> MFLIHFVHYKTILQKYTFKFKHIFLSIDKYNSLFFNISGILIWLNIIHINIILIKYSFFILINNFEYLIILIST;> MFRLTAASQKNLNSWYTKGTMRGGVPRIYYAWMRPGSFTRRRFEKMRNPFVDLETGTSLYFRDTRDSAEAIAHAADSKGIKGMDNAIDLYNEYRIVPDLYPEGFQWKHKLNTEYNQWRSNTWLTPDLIPKEHRGRFLCNFQLNIVAYDMRVVKFSPKDHRQWIYCVLYVGSGKGIAGWGRAVAPSTQEAKKEAIREAFSNIIAVDLEQEGPMYPVRVNADGVRVLLYPARRIVANFRVADILCAFGFQHAGCRINLKATNNPKSPTHTVEGVFEAVKALRSVSEIAASRGKVPHSLIYNIYPYLEEIRRRKGMMAMHPPGKDGLLMPDRVVDNRLPDHLKRGYYDDVYWKDFFAGSDEHLNEPRMGLRGDEMRRRLEEAQTSPAPTTAKDTRRRTLEDVLKRLGKTTRDLGSIPIVNPRVDVGLPTHIKRNYQLH;> MVFYSFVLVMKPRQRRFTSQALREIGVAVYSNGGLIRSITNEGIMRPYSRFRDADNTPLTYARYIILQLDMGEEEMGKVDKIIREHQDVLMALKLNNLERPVGIRSGNKELQAAYFPLDTFTRLEEEINWSPQTSADIYTQLEMNWKEFSRTRWSSFLRN;> MLRQSLLSLAKVYGAVPPLGAAQGHRLLHGKREREGSLFAVANDVKRDERLLRQQLNALLEEERMPMQARLQRNEAVSSHEAVPQTPLVDLPGVERRRDLPADPITRLFFQHKGDHALYYGTYDKPSVQDDDRVQIEKRVPRRREENLYTPIYDFCHRIREATEQRKRFVVVPSTIETRGCARVMHDHGLVAGFRDFHNDRAFAVELKYFQGDSTINVIEPCSYDGRTEFEWSPKMMRRLLNTHGIHNRLVVYICRTADNRIIDHIHAVKENIGGRGLMMVH;> MQKLLSPRTARHARLFRLAGKLADSGSPGVPKSDGERLVWVNSHVRRDKDISLSQEEERIRELMMPLEVGENSFAANGQATHGNLFYFREYPMYPGEYVPAEHNTLSSLRDELRLDLTAQSLKEAWMRVSGGVYFQSVDEYYASVDGLDAEQIGEVLAALFPELNCYEAQALVQRTLECISRPVSAASRQLSRTITAEAVGLDNAPGHYTNFLEWMGRLTETRAFKTEHALFEFSRRKFNRDDVRVMFENYRLMSKATLLADSADSYSHFYTVLKDFARKVAGEDSRHQIGVRIDEAEVDPETGIAVGRGCADGEKYHFTALLRENRDHNGIITVMGKPLSLVLDNKAWLMEMVLMPFDEANLDYRDFDAHIVSEGHAMPSIANEIAAFALRMAVANALVKLIPLTRIPLKKSGLLSVDRRRERGQFPGYLDGKKVKRRFAKR;> MVRRSHVVAYYWSRYRMPTQMPKFDGPAPVAAPQSMNSTKTNEFIDPIDDKFPMSIRGPLVRPDVPEDQYVDSWYICTSMTHHMGDYRPWSASAPPNAFRFRPFNEFDAKGREYVQYMREFARFDPRKSRGNGQKGFPFRDAYLTKMNEANQKTPPPTLETIMDRAVREHHQHARILSPLEVQRDVGRLEPIPSYAGKINADRSVFPFQWKTEDWYEYEVAKVRNRRFVFENTEEDGIRGSEVTYKIVLEGFWDHHVMKLAEDVCMFLKDVGRQIVEEKLVAVRRLLQGGAVDPELLAAFNCARAGPFGGLDEYDKEEVANFLRSDLRRLEEQCLSVINRCNVPVPGATNIYDPHTSWPHVEKLEPWVRMAEFWTSSSDTSFTELEMSTAHYEFRKFFRVIICKLPFQSTEFEKRMYDIRHWLHRQTSCEFHTIYRRNVIHDSAVFPTEHDPATPTTHEHHRMFSFALDWQSAPVNRLSTDTVHEGESWDAVAQRLGCSVGELKDANAERETIEAGVVINVPVTATRRLTSFGATPLVLPLKTTSAKDGERIRTWEEAAAILDCTVEELQQCNGHAALTYQKKESEAGEFDSSVTELVAPLSCWTSTSESEFSPVERVHANDTLVAIARRLQCSEEALRAVNDGITDVSGLDFVRVPPEARRPRRLVEPQLRPQAATDALLARTIAEEETFKLKSIPHLPQNAERFPHEYHTPTSRFPPTPSETPATQDWMAYTAKYLDKQFTISAEPAPVYNVNKLWPMQQIPGKVDQTPFEEDQTWLLHSIPVQQLEMHHHEKDLQDLPFINHEQFPRSLEWNAP;> MMRKSVTFLRRGKPRPRAGMFPDKYRRVPMLLKPQQGGQQYFNHFLIRSTNDRLTQQDVDNASGQAHSFISPQLPQMDWRNMSARSSEESIREEMRQLAENDVMQHQRVFNERMWYEKEEEHRMKARSCPEETSEHAXSNDGAVPPPRVLGGDYFKTRFGYSLVKNSEMTQGPVDYSQLDMWGEMPRYTSDMVFLYLVSRRRNTYAVAYTYEGKRILNTYTAGNRGLKGGDRGFRSEGSTDNGHQVTSMYLNDLLPKLREMRASEGRPMGRGEKVELVVRVMGFYNGRQGAVRAVQDRANEFHVRYFEDITPFPLNGPKMPRGVFK;> LFFLRMWFLYGCCLRFVLFVLCYYMSPRLPSSGNRRVLYAVFYLYNFVWMLRCFFCCFIGLVMSLFIIEGGGFVDLPGVKYYTRIVS;> MFCFSRGLWMRHIGQDVPKRHTHFVLESRLMYEKSFRDCWLHSVCRAISQLDEPLSKTVVGTHQKMLQRKVTCFQYNQYGLFKTPYYRLANVDRYHAVQGVAGTREWVPYVNVSYWTMNKMVRGGNLLVHRVHYTGWGTDSHLKKGGWEHRWNKVLQRNVLQYSRI;> MFVRSFCFLRKYGSKSKTPDLKTSFTKTTNFRKAEKISITTTDGEIVKGRGKIRRRTHSALKEAIGAMEHPAIWLWYPWRMNPEPPTPHMPQRRALKNVHGAVFNDLTPVQKKRQEQMLYGVNIPETRQMKFEEQHPLLAGALRKLEGQPKGFPFWYRKYPTRRHAYEYRFSIPVEMLDGYNDDVKKALSKGMMSIQEKQFAQEAMYMERYAEHDFDTTSPAVLAVKRALKCRVLRNHLLTNPHNNIIKTVLANTERKLNHALRRLRKVDFKKYWEIIRDHDVQDILQPPNLVTYRQGSYWKYDWNAGLAISTNLADVMDPRGLNGCVETGRSRSEVARDLGLSYTRPLHENEKKQLSHQAVYYERLAKFKMEQPEAARAMERERFVRKFSGMFVKMDIRSGAPDFPSTYRRLLGTKVVRWASKRHGPN;> MQVTETVLARAVIKRRSPQLWGAPGAPIIRMRGHHVVWKFQSYDLVVEHTHKRRNSDIRLLHYLGKHCPHPQKSLWSPDTPVAQDRHLFMLTTVDIDAFKYWFGVKRCRLSMKPWALLAKAGLLPPSLTQNSKIMPKPLFDKESLMRYYLANRKDEDVMAREKYLNYENSMVKTEEERAAERPVAPYL;> MLRRSLLAFPWWNFQTEHRQRCVLMYGGARTKNTHNANHRVFIKKYKRNAFPNRTRHHWAVSMTGVLSQRPRRMPWPYDLTSLIFNQPRQGSDKIGYVVGTSMLKTAVVATNHMVYYPKFNQRVSRTKRFFAHDEDLACVEGDLVHIKQCRKISKYKHYYVFSILEPNVEGRERLKLGLKAVPPPLFGYPVSRRIVKLNLTSTEGTQEKLAAAIQEHVQDAYRFSGPTPDQPRNRLADPVTFEDANNMIAPNAPAAAALDASDSPPLLDRGEYTEVEQDTRNKKGDDYWMNLQPKEKYDFKSFKKSP;> MNRTGGSIYAHALSQFAVCRQPWNEYIGLLTKQDSTPYHTEPQEKPAYRGRKQGREGWLFGQQVQLHYHRFPDEQLITNLSRWRTGETVGDIAMQQFRNAQPFDIEDKDPQGVQRPSPEVYMKLNYKNPATISRFLTRTGHMYPADILPLNPEAVVKLRVAKAQAIRIGLYPRFGNPFWFRSQKFRPKAYQENYDPTTYSTKRTVEHFAYNWVQTDRIRRYFRELEAVHTSGSASARGSGGGTTAEHKQQDQFYSPENQPISLHRNNISYMEDVGRSVKNPTVPGLMSTKGMKKKFHNLYSSTSTKRMGFSNPTLGIKKV;> MAFRNTFTTPGKFSTVSKNIVLLLIWRVKVFLRAEGFAHSLVMLPVSLYSKILLCDVKKKIVYFHCCTRKKSMLRRCPCVWPDGPTKSSVSIGTAFTLQKRFLKIAKSAFGFYLARRGQRKYPFLRRPHIKNTHSMNPSAPYFWSFMTAKSQMAFLPEENYITGDWTGKFFVSKRQVYTLQHATSGAKVRVKSFPSIFEFNSPSRWNIGKEMNTLTKPRMDLIDEQMLTKKQRLDYVRAGLLPK;> MLHTTRLWLGGYMMYHRKAMGTMKYSKWKGAHGGISHFYGRTPMVEEVRPNEPITLVDRRIMHYVHHSRLRHFQLFRSYQEKSNSTECKLREGEMLRRRWHRRLQKSFIAFMQFKTMKVLEDQARLVNTYGQAAVNAALGDPWNATDNVARERKSAAVRRQVRALPMVNVVPKHVATMKQIHNDRFNYRWRVN;> MLRRAYIQRRYPFNKRGPREHKSWKHHVLTEPPKPLQWRDPKVWTRDLSVMKSFDAPQWDLWQSRPRSEDMDEALQPFMDMPKSLKDRRYDIPWWANPFGAWYLQNILSLELLKLKSKTNAEKIATYRSYMRSLASGKDNTMSDDDVIRNIIKERWKTLEFGDRNAGYPCTFGDYIQFLNEWFKSLDEEGMQRLREHFDRRIRPLLAVMSPVDILWLEALTQNSPHNKEQLQRKIAFQTSLGTPEFFDMSKRLRYEINEDYKVRDELGPELFALWSKAPERWPPERLSKMYGLDFTLVRKILVWHHFKACYDACVEPDWSLPKRLFALEWIRDVRARKHGLFYGKMRFAEQKITFYSDRFLFRDLVNRREASYANVWEMDDPYRFLQTEQDYEDYWGDNYDVYRRMFPEMIGRTGEPVQQYGQMPIWAGPHRQHANKSEHNWMFAEIGVNVGHEALKKLELDPTNEKRRRFVIRQPDGTLRSAKMSEMRAWYWKEEWADFRFWAPQMEWGIENTPSQEQYQEHVPDTTDADFRKQRRIQSRPVKWFYESHYTRTGSFAGFQPLRFMQRRTEREVRWPDVINAAVQIQKRKPAAYIFKAIPEL;> MRQCVVRRYKMPKNMGVAPRFDTWNEKYEPWEHMKRMGRLVGTGFYIPPEWYNHFRMFPPINHNFQQEKTLNPHNASEPTQDDTSTLSPERVALRDELARKSRLVASEGMRYYNIFWVRKPLDTMEKEYYELKRRGVDHGEAIRKVLQGFYSGLAVKKRVAAIQAEEAKLTGRFITMREATVVLGVLAKLHKEQLTPHQVSLLAKEQGETTQSGAKLTAIVSRTQPHVNKEASSPATSEAVGSSTEESLSADALASMLSEDGEQSAVGTRYQVEVKETANDSVRQLREKAEDQTGFPDWYTGESPTYSGTSXCSRDGFALMKANK;> MMRSSSFCRRQIRPYYNLPSKSEHGRKMTGFLTPYRHWMWKQNELWRNVHEAQFEHLRRVYKRQWLESFRVNADEYIYKYNITKAAQLAQWECEMKEQEKKRIEARQMMDGRQALKKKHLDLLREFHERQFFFWYERASERLQNMNLINYVPHAQLREHIDKELDKYVAGKNEPYPLNFVGQMPFLEDGDGNIVEVPESLLSNHMAEHPDSTAKPHEPHTSSSISEAAAFEERMLRAMVSAKEEDLKEWLGDDSRALSETIDDISREEEEREADIRVARSMEETDAEREVSRRAYIERXKTGSRSIFRPPTVSEGAGGTPSAPAGDANTPMRRRKKGKLDRVHALQAHQDELLAKLSSQGLKEXVDASSVPERGKIVQSRGRIRDKAVIPTHEVLMQKPELAAGSTPGARIQTKDMVDKMYHRGKYKKSGSGDKSDGEDL;> MRSKTLKKSLAAMYMRPPVTCYTDACEAPVAMWDGAIPLKETRKLKNGVPVRTVSRTYSHPPQLTPTQLSFNDINSMYCVGNDELIQFFPEGLGGRVFQTMPPGHPRGFLYRKETHLLNLFVDKVQHWHTKRSVLSSLTNGRTGFIVDGPTGCGKSALMCQVVHFARSRNIVTLYVPDAKVWTHGEWCWPSTILPGFFDAPDAARSFLKYFAVANRATLTSWKLRCTPKDLPTEQGERQPQNLYELCEWGHRAVAPASIDRQSVCVKFLMDELSEEKKLPVVIVVDGWNLFSHETHFRYPHPDFLRGLASFNESSTDIDLYPQELPRIPASRLSFVRGLNKMILSGDDPNKFFITCTTRDFKPFDGISGFPNVETDRFANSLDEYAPYDPEKDSHFHPIQIGNFDEYEYRSFLRFLINSGELAGLGWGPLWHASSDFERKLYKIGFLSGRNPQGVVDHYHQELVWRYDYQRTRQKQYLLKRRMEGMSRGASSGAVGVR;> MVLRRWFPLLGVHRVGYTHPSTLPVPCAQRWDLRLARARIFQEYIEEKAPGAWQLEDERSMSPEFKTFTGYPMRDMRPGYGQNLPDYIMKKRLPNNTHYELFARRDIPNEDNAMYGKYLYDMTVHGTSLPSTYRMHKDINKAQRNDRKLSGNRFKVLCSSGAKNPPSGWEPIPDATEEEED;> MLRCARVALRADPLNGGSSMTLGSKGSKLSPEPHRRRMPWTAAKEYVPGVVLNARDKMVLDGVQLLDIESIDRASQLDPLEVLRAVVATREYNISTGKNIFQLASQATYNGRGQRFYRKEWQEGTYDKYVTLSAIDFDRDGNKGTAYGYITFHGETTTRPVQVDFADVPGWYMDFVEERAVPFTGIVPPPPSIGTDVPVDPHSYRLKAYPYYDAPNPPEFVERLLKDRGVLPDTPTETADVDKDPTTSDGSVHYDGK;> MRRWHRSLNPALFGERGSGHYFSTTRARLQLQAQDRIICGTHGAGIVAHQTAVNSSDNPMLSSVTTAAPAADLSRTKPHEGTGTSERDPYIRTLHNQRSAAPESSVSQSHTVNAPTVDECEMLAERWGTMNYWHNDTFPRLVVFLKKLLVPDVSPLSPTAESLLSMFEKVVIPKLTSDEEDRRKLVSLWSETTLQAEAAVTKFLFQRGSFESMLHRIITDALEKMSTLALGGQEGNLALEALKRQTLFKRNDYIQKRLIDVVSNSAYLGYGDSVWQVFFAAVEANEENLLSDRATTDAIRAAWEGVMREDVVRLPDVTGVVALYLTLVCIRESGRLVPEELKELSSGLEDGVRPGVRKLQQYPLIFLHPTVKRRFVVKAVAEILHNSSSNAFSNMLRENGLHDTAREVALCEAMNRNKELAEGDVGDAVGRFVSKGEVKTLLSSLVSGTDAVVRDAVAGIFGIGTTITIDWDAVMQNVDWSNNWQRLATALLSNSAVLSAIVKLVKNAIGAKGMSKHLFTDEYADQLQLILDAREERAASRKQRIENIAQELSSFERVDLSCDLLRKLGVDMTELDTAAAATRNMNVVQRPCIEDGLLSLVLEAVTKRHPNWVKAGVIQTTLKDPFDALRWMMHIFIRLSYVPHAGAATIARLSRRRIGPIGLEPHQFNVPAELGFVEQYDNLQYKRYDWQGWYQRMLDVHNRNVSLRCRICDLQRLDGNGVQFVDMQTERRLRILAQHRVGMGVLKLDADKYEDQADNVTFGTTKLSELLADARKAQLGEEYWPSVELKVRKPSGQSKAHYSLIDNERIEKRSGELYEKYRDAKKRSLFVTPMETWLEVKGMQVRKSVDNADEDGYTLDALQDMMDGDDGDKV;> MKSSDIFFAYRLTPVVFKSRQHDSGVNQYGLKPTNAYDYINPTNLINFGRGTTFDNLGVRRAGRGEIDSSPSHSGSPVFTQAKLIGLSGEEQLTMCQSETMALRLCMAKAGKETCERESRALDSCLGRVGHLRRAMSEACWEFNDWFIQNVSDNHTKPFQHRPHDWRHFYAQEKLVRERQQNGHAYGRRPKQFSFGARYVKTDGYGKRPRLPYNK;> MRAGCVACSRIPKLGIAALGSTTTSMQATCQETQELRCATTQMAPAVIFPLPPPLRGSYIDRKPTAASFNEHHATASFRHHMIASADVSHRPRHFYFASGTRNDTGTRSVKEGERKQLKQQTNVEVDSVAYGDQLDELSARWAAKFYGQVTFGPRNYPYPSSRWLARRFQMKKHRIIKRFRFRRYKLAAVANLPFAKMIRVGMLPELKSSKTKRGDVVDPTLSGQLVSAVKNTGEKRKGQRTRPKSKYQV;> MLKRTLTVLDQTYGPHKSYKYTYMPDPRKLAPIETTQRSEIVPQSIRPPTSYVPNHETFLERADIHRLRPTSDFKASFKDWNDLFTCDKRQLRVRGIPRMTRDAIRTAVQAFQNGNPPERFDTKEEWLYYKQFKTVDYSYRVIPELPEKYRPHQSGIDQAPLPDYREINKMPQWAECEERRQSKKTV;> MRLCRRLSYHAYVPKGASVQMGETFMPSNIATAVFRETEAAAARADKTKEETGFFSQPRLNYPVSSGIPALFSKDQFDMQYSLFHRDVVETLNRHTLGTPLEGHNLETVIRKTSFDATQAVAHTAASEHFNYCFFYKSLRPWGTAPPPRLREALQLQYGTNGSADAMDEVRRIVWVTAASHQERCGWVYLVWSGVHFDVVEFPHGSCPIASDLIPLLALNVHESAYILDYGTSGLKQYVENYFKACNWPLAERYYLMAIGQVV;> MLRRTVTSLRNARELHRLLPALLPLLDPPVPTGASVCAAHLIVATGHVSKQREPHMSNCPVLERKIPLSEIASDDNFLKHPCVPCLKHRINFLASEDFCYDFVERCGCGTDGALPPEWRCIVERQFGSMAALVEELVIHASNRREAGWTWLVYDAQQAGERPLLVVNMPAQRSPLLLGLWPLAVVNVTEAVLVEAVRAESSGSVAAAPPPPWCRAARASLYDTKAAAEAFAMTAPMSEGVGKKLSEIREKVARDAVSRMNWGFILQQLKKAETYYASSDRGEKIRVHRMKLEREAVTKAMSGLRDSGATFLTHDTVEVTTTPSANSEPSSPERVPGVQAKQPQTEGMDPCKNKASAEPDPKCTQLPDGTWQYSYRNGDVTLLKPDGTRVFRKRELTTTAYPDGSMLFQYANNTSILDRADGVRVTTFEDGTTKEEMIRR;> MERRRLLHDGRWFTPPVLYGSARRGLKTLDVREYRPLAMPIEFRFYQRYANHPNRQSGIQFLTHYNTHQRFRVNKDYIDYMHWGKEQGQARLPHRHQRVAFDFNDQLHPTRIGTPEDGGNANHCYPEDGEDGSYAWFASQDPTFGHHPDLSSSFDPNYRVFSHPEHWNKMFTKRRPGEGDIDLSVLPSRSLLGPLMAHSDTKGIPYFKVDNRGHSNGRVPGVNAPFFGEFDQKMMQAMSRPLNANRTITGNDGRFSKTIMINEPQCNQALSAKTASELSKEIDKATNAVYSKLSVLEAAQSGLTDYFCGGLNFEIVGFELHMAAMLRERAAAILERSGAGGLPSASSATLSSSSTTRRCAMLLEKADEREVNKLLRDASRYEDRVDDALRQHASLIWRVYTAPRPLMTLTNGKCRGTGCGLSLFAKYCALKDSSEFIFDGPNVGITPYGGMTRLLARPETSLKYPGLAEFVVLTGASLFAGDALRLGWTDLFTTIPDMTYHIKEWFDTTEHMHNDAVAWQLGHLLETCFKMKESHSSAMERAAITPTRARWVEDAFADQPSVNDIMRTLTEIEQLPFQSTHNTSDESHITPYTLGSVAAGVQRLGEHRLRYTLSPWDITPPEDSVVLKHTSEMFRAYVLERRGATDVVTHRDAERAAAWSQQRQREYDAYCSLKEAPHPRHVYARLEGCEGKIVSFEFVFEISCRRSGPQGTDEVLQATTISRLKSRILDALGMPRDRNIDLGWYLPTLDTCPIHSDEELMQVLHTDPGIEDPKEKLRYPPIYFIVKRCTLYFSEWAYAVKHQLLLQSPFALRAAFGLLQEVRGDGAA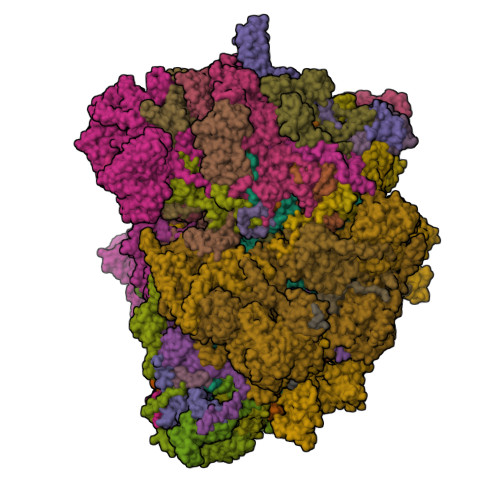ENVMPLAETLGTEFKYFTRLMRRPDFYRVGVHTDKSVEKWEEIKEERRHNIHHTHRPTRPLPDFEEVFERDVEIDGHRFVLRPRWNPRTLQDVDDSDILRLRAPLTYDMDSTAALHVPTHCGKASRLAGMLQDAGGVQVLDGLGEVDDKGEPKVPPLQSNASVPTNVSFYEMARHPWEDRASSWRRDGFTEGSLEYFESQYRSAERAVYDEEGRGVRNYWPSRDAVEGIAQEEENDAQLLQERLFNTLETAGTSVEPWARNLRLNATTGKFGYKTEIATQEEKIYDDEYYRWFIQPGRHPNPSGLTLNGRKGQFEEGHSRDEELERMWRKVVADGNNDFAATTSGMPVYDEDAKNAEDSYAAGDDVDVVTTDANVPVDGDDSS;> MMRRVASTGSNGGHCYVGSSLWADSVYMEVSSITLQKRFSFKYATKLQHDEMRQPYYIHEKRYGIFSNERNIAKARRGLPFITPLYTKHMNLWDTDTDASNNRFFRGYYYGQRELHQLLGRPHSLEATNADGSNDLSTYEANTSQLYKGIPRPAITNLHYEPAWRYTLYQAGAHGAQLSNPRSPFTAKVLGDELMQVRDIKSVEHCKAWFDRLQYLINLHYEAVGDIGEFKSRHTRHVHEFFVAFHDALSSLDFRDTYLFDQFKAVRPPELSDLFGIFLEMEANYVHEDYCPRCSLPYSTTRYCGEGDVDTPFRKHRGRWAPHQKWGREWYDVVARRAEALWYRATEDPYFGTPQHTQRQAEALLKVYVQAKQRGKAIDFMNKLRGSVEYLTGDITITTVMQESYDALLDTTPHPHLLTNGFTLESDAAKYTGEVNKAPLSPLQFRIDMEMNKYRRQQKEEGVVRVPPALWRLDTSAIVPYKVDSKTRRIVNWREVKEGIEKSFLSVGLPKEAYTGNEWREMLYLHDVIANREAKAAVLEQQQKLDREKLKARERASLKGEKSSNSASNGIGIIFPDKDGYQVFFVDEASLRPFGIGASGTLFKAVARVYPSPAAVPYDDPVHGKQFLIDTTDETCHLFGGFEHGDRLLLRAKSSGGDVDGGNNSNCRNTGSFTDEEEEVIVMGVSTEGSDAERMLCAMHVDTGKQRERGIVFLGTDCIDIRERWESVRYAASAYVKGRVTLLESQRTAREEFMGQVVGIRDGVLFVQWRLLKGGGSVLDRSVAVPIGDSTQVRELFVETKVLGVEPLQSPPSWRTPFRNDFAEERLKELQRAPFKREKYVSLIQGKYTPKVKKFGYTQHTTVDDFETKEYKDRLLSKQFFQNPQAFEVVPDRNERSVQFGGKWEYQRTHGLPTVDRNELENGWSEVEPISDGEMKVIEQALRDISGPRPGNFVKPPSKTKSLQLSESWWEPLGYGWEQHNEEQKALCDVTEQRLIDGSNLPFGGKLPPFGTSYGMGERMRAIIEDYSKGFGLGPHGHSPTHDTIHYNTLNAEGERVRDLGYTDALGRLFSEKLGDRDVHQWAVESCADGEADVRQLLLSLHEWRERGRPPSLLLANVLSKYLEEEIAAFNKGIPENAPKLQLETSDGTLAHSGSGGSRSGTMWADVDPTTFALHQASQSTRSTRCDEPFILHLVKRAKLGECVTNFTDTAYIAHLESSVINEFHLALTKLVGKGISPTLLAQKTGQLHRGSVRVGGNVVPFVKSRELSRLLERMGLTSESIAVITRGLANCPEQESVGDDFAVPVSLILSWDGPGSSGGSGSGDRRLNTTAARNEQQRKGSAALSSAIRQLSQHQKQRGSASGRGWQNEDKMVVHVLEELSLRNDGLVMDIQYAIRENKKNRRLRWEFVTTLLPVFGGNEAKVEQLYSDYCDGKYVPNITVAVEAFIAFLHNATQHPETYSASDYFDIDDGKSSTASGTGDQPSAGQYTTLKLLDPLEGPFVFDNVKVEYIQTVERFRRHGIRAGPVMAPATGFIAANCKSLNYFTRRQEEVVYVTNDSDQGLRRSLENSAYHKTIAANPALQYLLKARRGAALVETFNRFFYRTMPMLNFYQNVLKHYSETIQPLRQAAKSSTRGLARALESERSAAMEEFRRNSERYWRNIIEGRSVEQVVLANGESNRRTVGGGAGEQLQKPQGNRDAVRTNFTGEATDGSRKGQRQHQQPPLSQQQQHSRGEGERSAVHTSPRQGGSRGMADLLSKLNTPKTGSGVKGSTAKNTGNNRRGPKS;> MIRRRVCDGARLAPNIRATFSAVRYQSGLHTFIRDSKPSNFSSVRRSENANGDATASPGATAGENPASSGDWASHMQRELFGEVDPLGGQAHKDYYRDVTRGYSPQYAPRNFANGGAVAYPHIQSPYEYEEAAHRRVWLDHDVDRMREEFTQHRASLRSLASAQEREELLRSRAAEYQVANTVHESESVHPIQQLYNSGGTSRSALKQQAVADRYSIAEQHSPLPLTTGVDRDALDEAQRTKDRILNDSFTAENLLITHGLREKEKHDFTILQRTVRIPFQGYDMDRFLAQQKGTPYGAQQLPPNVVPSSMEEAQRTLRGSSATATPLVDAVAQKVYARNTVVDRPAIGEQLTEQIINIMRASRTTAEQQREEERAQRFGLGRQGALVQDGGPDQRTLKKHTNDERIVDAMLFQQNAYRKTPTDEHWNPYIRRSTENGVGHLLQNKFDIMRREDRLSKGEQDLTERNTIHYGVPIQQIVDEFVFRHRNARGERPLDYFKPFPNFRALRLNRMYRDVEGFSLMKQRPEFLEWELFTRYRQHHQQRRRLALLHGLEPVANETAQERDTRRHRLDEICERTPFDEREMRVNDDEMRVSVETLRSWFGVYMLPSPTVVNAVLGGSASVNLHLYHLADEMGTADTREHVLSSRYLNRLLLLESYQNRVGRGFMNHVVGRAPEPVVPHEQPQEVLRHFSAEERAMYEQHVKEQTSRQLGEWERAMKRRRWLTDHQQYGHVVSHGLETSVVDLSHTETGAVLTVSTKAYEQEIEAVRMKTNATIKVDGMVYNLLPNSERRVVPLTVQLDSGEKIDMTSEDFDRCELEAFPRNLNHALNYGIANYAYNRGNYVETQDSIWEEQTASGQEGWSPATHADGLREGLPVRARRPIFSSSAEQRIAGGPQRAVIIQYHHQPFFNPEPRLVKVAFQCDGTIMEVPISDVMIWQRRYHGPERTVGDESRRYNPAAMRRYVDVTDPFNEKTSNTEHFLDKYEPKRNADTVADKYRTTKQITEIDKWTRYDSARADNYRPLSISHRRDYIRMGYIPRYTPWEWIAIQEADQPLIAEQIRQDNIGTSYFFSLNRYWRYKASPHGYIRHFENEVRDLLQYVDGVTPWKQAQKIRTYWEVRSHHPMPQFNRPEVAMHRNTVGLLPAHMWETDKKTGKVKSVKDSVRDYQTKTPYPKWVQL;> MFRVRRLAGFIQCSPCGKMGPLKQQTRRYTPIWKSDPAVDNVAPLRDEDERRALWAEVGPISDVGSAVTAWIRFGNDPVLHTAVPTMLGGKFRNQQREKESLLPNSSSPFAYVEDYMGTNLVFGSPVHAKESAAVWATYFERRYASRLRLSRRTVANYVGLINSPEVFDDESDRPETRWSQDTFFRECAYLSEKFLKEKVSNMQQFEAALKRASPEAYLAFFDAFQQQTQTQIPLPSPSVWHYEGERRKQWAEKFISISHKAQAFFKDVLSEDVKKYQEVPGKLLQKVKPVLADVGKILVKRHERWLKGRVWTSLTEEEREAYCMKEVKRQQMQVEDGEFDPMMEDDVDDTELEEWQREHDAIMKLMNSPIDGLHFTTLELWLHTMRCEELETEHIYTSARVRAIQVAARKKLYDTTSYEEVIQAVVESIARGTLDLGAGVLRPHFNEVWCQLNYAKFGSSTITQHTTTSRRQLLFFHAGSLKDIAATATLYYATKPLSNSLDYASPYKYRRSLITLCSNYGVETAYTTQRPLLRSAANLARAEDLIHAVVTAAAQPFGERRRAATRDLHMEFQRLAVPVERVIVANPVSALLESGADPDEKPVEGEKVNMWPLGAKRVVLYKWSAPNVEKLKAMESDAASAVSGSSLTAKRLREIQELKRRGFLEVSLWRRVTAQERKQRNEIVEAKKKQVEEVVRTVPSLAHLHQYATSLYSRIEERVAFPTETSTVTETTNMKEETNKPLEDSEWEFAVLLDDRVLLNKEESVELYLPYRDANGELLAQGEYRALVRAFDLEANPNLHPAYCSVGYSESFQVFDALPQLIAQFFRVKDATAEAAGVTHIPAADFTPFCAFLRDAGLDVPLRCEFEAGQAVTTDGDVYMDYFLQLLRGEAFHQSHAQAGLTEAQRAIEPLCRAHWVVHHPGADESEWATARRSVLDHAMQHEREWWFPNEMLDVKDVVTGSTNGLTPQMYPAAVRYGVELCTVLTAEGKFVDERGSGLSARCVVNGTGAAESVVFDTANCNGTNTTSVEDALRVAHGALRSAQDRHNTLAAFRLGPLSKQSQVLLFCGVNAYEFGGKYARTYAYAFEKAKKELEATAASGFMAPSLSHEDTERLSDQPTTSPSVDRFASTTHPEQRKAQFVPRVGPGSTPLEDPAADQKSEWS;> MLRCTVVGHHRSGKARAFVFRDPSLRMMRAGSGYQQLRRMGMPMQVGMGWRKVDSFHANTQYQHAWPLLSHDDLGNSDQSNNTKNIMYSMYMPKRNKGTAPWFRGADTYSVKYCEQGRYEYQRYLMINRFPSEYKKHFLSFLSNIRMSSGSATIPQEALHWLLRMIVDNFNPQHVHYIAAMKTLQSAGELDMARDVWKIMERQQTWPCTATICAYLDVCVEAGEKTWAMEAWNRYCTELKFLEPGEVDPKPISRVPFSLTREELLYLPKWKKHFDHDPNLDVMDLNRFNRTREVYLRMAQVMLAGGERNAFQHFFTKLEEAMLNKPTPVPEPPNPHLVRRPRWAPYEHCKSVHHSPWRLQNNGRALALGPPVTIEDEMQSRFFSNDQFLVHSVKEVLRIVLQEHKRAHPTECTRCKTEAFFYKTKDADETLKFCDDLIERLFASLGVRLSNLNTSSLLSTILEVFRVVGKESGAALLQRANEFLERKASLGDAEGSRENLTASNYLQVLSGFADESAFVYNTKKDGTCQYKTGFDPRTTMRHLADVVQEIAGNPHVTWAADMHLQVVETMVGCGTMKANDYFVRNVLRQFSWDSRFLEALYVEYRRQDDVDMWAELTKRALVWTARYNAPASERLRRLIEDDYDTIRVQTRTFRELAVFQFRDVEERRHSRDVVNELPNPWYDYVAHALPFPDRDAGYPDEYGDLGQWRAPGGPGSPVRGPGYYAPPMEGEHQRGYTAEWRDLRNPMRPPEFPTPWERKYRQYARGQHPSYDMVYAGPMPEIFPMRRDFRKPTRWDFHDIEKQGKYRTSGPY;> MRRCSFASTCRYRSADDVPLGLGSAYVWTCRNITSRGQFNPIHNFSYAMERGVRARDVKAFEKLITNPGPLRVAYTPDYLDWLHRCYKAKGTYMDARAVAEKKFNGNIVSSELSAAVNRREGKRGDTRGDTVDNDHHNLPGAPPPGMFLRPAHSFRRLAGELKRRRAQSILDEVARAQGMLDLFERQPHFPAIHIDRCSRFHLVELFKEMVLERSLDSNMIWEKALLYRAILSERKPSYPTSFHYIFTAVEDTVFAPTISTPMEMAGSGGEGHDRSSHPLAAKCPTLEAYYYYVYLVKKYYIDNAVEAHVVLRCHREPNAADLLFSNPPPKDDTEIMKAVELLRNADIQRGVAAAAAVSDPTLPPGGEGSVIGNSDNXKNSEKXSEGSRGRPARPPVLPGAYPPIDMLWRCEENLPLLKVLLFGEFNLIVSENPFVKFPSAHGFLTRPYSTDSSRTLADGMSLANVMAEKRGHLLPSLPRNTATSIDARAQDIRRLQQKHHRDDIVSFQKLLRSTHAEDSPSAFSSYSDWSYFNPRAVRAEERDRLTRKAVEALKLYDSATNDIYRHSFEDVQACHTQRVTERDRTMPPYLPTLPHFVAIIKKDPHISFLLHIGLPDRNSSEEGSAKHKELEKRIYYLARALYHTALEYHNETVRRVNRQKVNVAASLLDNFVEQEWTTILRDKHDVTDVTKTLNDTQNDKKQLARRLGRYMLFANRSLDDTGFPTDARADDYTRWMAPPSVGKVSL;> MSVSGVFSKGRGIGHEATTSILRYIPRARVPWQPSRFGRENLTAADMARLWSRGRYRDGPGNYNSGYCTERTHVLEENTVSIIPRRELEKYMPDITIGPKALVTPVSLMNARNGHRVTHDLLHSYDPHIGRLGKPAVVDHDNITVEDPNRVGLNAATLDCRGRIYRWLRRGPFFQVDNYFRRSVKLNRDGTLPTDFVHEAPLMRKIIRLAHRGHLKAACEEYRRVTTVPPVEVYRALTACCVPGAKLADAVSIFEDGDSKLFYVSRDGEVLHNLMRCAIAARHRARIMWVYNVMRGRFYENVVVRAEVDLIWRYRIAMIALEYLLDHECAEEAAAIYSYLVEEELLRCDVHVRVGLHMREAIAAGKPITLNNDVMNATSLVRDATAVAPEVARELQRRHAQTLQNNAVEAVGAENVREGSAPWSILGPLTAIGPTAEDTMVWLQQHYGDVDVMSIMRWARFRKGKDLMAKDRPQYLARAAAWIELLSKRNREMEEVPLTYMRKSKPLVLDTNSNVRVAWQTPLMRSGGPPRLLAREEGYVFHHSNSSRFVEETYRHPGESLQSRYLALQPLHTEVSAKEDFQRLYYQAQKHHKQQERLLPVSTAAIPSRIVHHSVMSALHGVSGKGEPANRSLFTXNKSNDSHSNTGVASGTSACTDGAGSATPEF;> MFRRAIPLLSANIPRSVWDPAQHNPNWSDSYGHDITNRRAWPARKWTVGLEPCTPREWLQFSHRNLAYAYNGALRACHSLPSMLLLYKEMKQRGVKVDVDTMNVLLTRAARHEHIQVDDVFLLFDELVALGARPDLAAAETLHTVLSHSASMPEEWREARRLQLVELYNNLAMEEVERLAPHRADRLLKEQMKRFRGNLQQLGSGLRPTVYCRYLHTTHTAAVLLEEVHNFLWELVPNDHPAMEIPALQLRVPFVASVLRRPSVNPGVSLASVSRAEFGDTDVCAVFLAAAERMVDADFDDQRPVSERRLFLSLLTMISYSGVLYTSDLMAQLMEMVKYSNNDETRDSDAQRVLRYALRGSSAAQDSASRTLWHSVEKVADCRVVGRYIGARNPWNPIRVCFDEQGVFKAYPISTTTTTREVSPPEGNGAVTQEQRASCVEGRTLEALNMRWDDVRRLIECTGVLVTPPSERCPQQQKMEVFTGMAVYLRTVATGRRYEGGEDVLSDGAVATSSCEQRRRGTLFAEGYDFDVWVRLFSLVQEVRHDMEKFMADHTLQCVEPEFECWEALLVTLRCALDFCVVQMQGGGARGTEREVVERLFRDVVALREELIEESRTRFGGRMRVLWLQEA;> MLSQNVAKTTVPSYYMIRTNLPHRKPQNQWEGVYYYSGITKRQRHLILLHRKREREAHMRSFNISRASVLQRLEQLSGDRKQESLPPHVRLDLAVRLAQHGLYQQATPIVDELHHQKALHAGHYALLINALACPRLGQRILHCDAQCDPALTYKLLGDENGEERAQEAYRWFDLALTSLAVDCGGRTQPSHFVPYLPQGTAAASHITNALMRTLLTCGYTHVAAIPDSVYDRMGSMGISPTISTYELVMLALSLQGNMVEAESILSFLRSHHSEHITVESFNALLLGHREARQFDCCDAIWQELVDRRWPRASPLTAELYLRSIMDHANTPTSEPLQSFANINVVEKKKVPLVLAQMDELGVPRTHLSRVLMDEVEDSLRKFQTYRSRFYEWGRAVKQFDFIEFRRRNGWLYDLHLMKCTTKQVGPLRDFNDPDAVQGAVATAEIPAFFNERPAWERPPLEETLYVTTNKERYDDVRGGDIYYDDTRGLHDRSPTWMNEVPETRYDRLYGVNHPDIAKIGIRRHLNVEYVNRKEVVERDAALMKKTLSSGRRLRHRVESSRTHRNAGSLSGISSTAGGGSR;> MRKFCHFMANCWNSARSHATYGAVPLTHSQVTSVYATDGGKVDELGLLELVEERIFSWKLNKWEMRIPPNLPNDQKELIRQEQENLKQILSEWRKCFGALNADILQISSLTGVPKDVVREKNRTWLQEEVAKLRWMGEVNKAALLRDAFMRLEAFGSRDFMFMERLCCIYGLARQGTFDEAFTNYITEDPVTNDIFVDERNPFKELVAHIVRNYSQIDIIYDFLGFNYSEGYRSSLRRYMEYLQCKTAENVRASGRLVTGDKGEHNILFDYCVSRESLVSGDSCQGIIDFLYINGNDVTLIIIASDNPWLRNRQLPHRRQMEGIARRVCFVLGIPPSEVRIRNLLLPPTYLDKGSIVRLNDIVFRLSNEQSNLLIPWLTNYNKELDPKDVDYTALAKTTNEEEWLTL;> MFRSTRPRSVGYTPVNPDTSPMVAYSQYHWHYNLPQGMERPHSVNRTFAAPFQSNHSLVNKYRGVWIEFDMHPAFSVALEPQLRKLPRGRTLPKTPAEEVIADYTALAPLVDDEKTRDLWLAKVFQHCAFQRCGGAMELWERYCHQRFTAEGATAKPPLSLVKSVLFYCNKTDNSGWRALFDRCLKDGWNYTPLFDTAQWSFMLKSIGRMGDEDGVRAVLEEMLDVQADLDRVEARSVVIALNAVTNADVYEFVKKYLFNFGERKVKFLRTTYSDLRGHGAGKLRIPLKENDNMYYHVCWHSSIRSPRQFSPRQLYFDYTPSTLGSSSHNPNAKIDDIVKDKIEKWKAEGLLPEDYVHEDRVYDRSAAFKNVARQEKWKKMPKILKSKRMGYTGDP;> MSFRYTNNLIGALKHRLLLESSYREIASRKFIGNCRGVEVVCSGYGTVLAVQLTDKAVWESFYRKGGRPTVSGGGDVSGDAETGTQGSATTTGATGSLDLDKLAESIKTALWDATRKIRSAKEAALHRSLSHNTRMRASADLKHWYEEDANTLRPLAFEALKHEAATPWMQLVQHGKKEEAAALLKEFEQKGDAAEATPTRVKDDRVKGTRTELSNREQPPLASTLKAEDSNPATIPIGSVHPLFTPALVQIEEAGGGSVSNEAVCRAQLWELSRDEQLFWERVELIRKGQVASIGSSHKRGYADEAAFAKDDTEEKVQLRFTQ;> MRCSCAFLDKSVFAAKRRVIVPIHPTPNFPAHFIKSAFTTDPLKEKQKARFSSGGEAMREVQDIPKNLEGERSRRDLASRGDTEFQALVEFIEGASYDQLISGRRFKKVYDVLSENDDMFIWLCHTAMSVLNPGDMRSRLIYNHLRILAESVASGEMTQRTAFRFFESAVRSPAYREIAKRQLEGGAATRLAGISAAADVMRRMGLTRRPMSSYFELYQRIVERSEAMTPWGFPPLFQFEERLSLEPRLKFFSRASQQSLERRRRGHVMTPHTTLHGRRIFWIPPTWNRAGRFLGPHVTLYPGMTPD;> MEVYRRITERVRGALWAHHGRLMSERQFHRILAFVYNNKYEYQIRFDRMEVVGREWGGRVEVVTTPAGFLKRVRVNPCVEDLTLYQQQQLILSAYANACADGRKLMEQAEMNIYKQFLKDLKPIVMGIRDNPEFYTVSENSIETIGGVLQTGDSNNLCHTHRTIPAAKARQPADEVRARQEWEQKWINSPRGQSWALTLRGKTYFALHGPQYRPRGAPGAKKETLPLDIPAPYTAMDEKRLLKKNWMAYLDNKHVAEVMWTRVKIADREKRQRLLQETGRAWHRPINEEAINRW;> MLCRTFLRQFRMSGGDMFVEYKVLSRDHRRSIRVEDAIVDPTFKRTVLPLGWLELLRSPSLRLPTGYFVEETVHVSLPNATSNGGKKEARPQKGGFASGSPSVGRNEANAIIAGPVVLYITGQSVPVVLNPYFVPEGTWDMRTRDGELDLRLGMDAIEQCTLFSELRPGGLLYGKLPENPNVRRNESLRATLGRYGMKCDLAESPLVPRPWTRMRYMFIDELQRGPKLTEFVGHNPRNGTPWRFSQNTKYFRIGIWRDTIRRNDMNEGLHAHSSWQKSPQQSVPEVRFLAPYP;> MRRFCTARVSSYVKRAPLLLPRGGRRWRSGAGTTADGGGEKEYIADSFESTAGSNAYAAMELAAEARREIHELWLSAETALEREKRVQQVAALIEKYKLDPSTPREADVSRGLGDAFDRLLLLCLPLGKTDAKGTDNLERLMHLAGRNGRELSVRTIQHLFARTDSFAEALAVFYTMRRCHVAMNMEAYYSMLYSLQRLEEEGWGQHFRNEYEENGAPSEQAMDFIVKGISNALLPENKPWLGRVMFQDRNVPDRRYDTRDFDELDTAWTQRYKSGTPAGAH;> MLHGTPVRRASLRYRRPYWMMFLKGVDNWKIYTVIQQPDHQRTEMLYQAWLGGLDRPYTRPKCMANQPLWLSKKRHMLRKERLDGPETPLEKYVLEWHKKFHSFQGTERPTPDDLHTALDLVERPLDLSYALQLLGQCRNLNNIRFAKETFLVFLEACLRVGRRDCAEYALEHAEPLGFWFIDEDHRRYLQGEQTWYKLSPLDNLYYPVEENAKLNEGRKPITRLSPATESPGSGTAISDGEPSTDVEGETTVDDEIAQLEAELAALEREGGGK;> MLRRVPRVLQKGERGLYFPINHRIVDHRIAPGVTVEETDVQSRYRRELRTNFATGETRQTIAPPWSARERPTHFFSLRLPSRNSVTLRVKEMHNHLLFSHQQCAPMLVSPTKLHITLGVMTIPENSREELVKNIQQSMSETFACVQPLQLRFRGLGTFDFGRVLFIRVVPEADFGRLERAVCDIRRRVGGVLGVDLKGNPHDSYVPHVTVAKIRPNQRQQLGDTIPQSLWADYQHHDFGDVTLSTVDLCRMKGSPDGYYHTEGAVHLS;> MFSESLCILSRRFRYNTKFPALVSYNKLPWEVVNHETPQFHMHVAPHYEQLLTLAASSPVPHIIGSKHIDVPREHRLRLLPGMLYLLDGDTLPGEFTINRVLDPTALQYYGRLSSQIVTVEAVRMLVPDDLRLLCNCITFKGPLHLPVAPYASLASLRGASQGGTTGSETGSNCFTLYHFVRPNRPPKELQLEKYYIHAPCVAPLSEFASNSDERGNWRPRLQAPKRTRRATPLPAYRPPQSYLMGLAERLAVVPGGCFGRRSLMWGHWF;> MFNRNFILRAAEFKQKSRWSSVWPNMRYGSMFLSYSVGRKLPMKGVNWVTRDSNRLLNFSNRYSAVISDIDVKRTEEELNVALSDIRWNDHRRIYWKCSFCGSSYRKNVSVRTKYHAGCNFCKKKYPSEVRGEQHGSPPVSQAAPELTEQLVDNGKRDNLATLAVTSKFYAEWTCRGCGGSYRSTIRSRTGQVEAGQCTLHPDIVAWSAYCPSCSWRPNMVPIAEEVSRSGQFLGLERSMEELGGQRGKQLPIPRRKRLAC;> MLVSYLRLQADRRTRHHMMVDGQINPREWFNWHPKEYQPWYFDRHKFLYEQRQYAQFHHLLCHQVYLKDMLHLMRYPEPYTHIIDCRTSTQKMHRWVPHSLWLPRDEVEYALQLSADEFLDMYGFRKPDKSDDVILLSHNGIYSEQAGWEWKKQFFQHVYNYRGGTNELFGESYSDMNVSDVLSPWKGPFPQSGVFVDKWSKRKVLTRTGPFDRQYEMQDFALPDLELEKARHPEEGPRQNMPFGLQ;> MRRGALSLLKAGLLGHYQQEAFEARKRFEESTTYPGPIRAATPGDTRFYSGSLESILHDTDRHYWRAVTDDPRVQHLIPLRIRFKIFTWVTSGWEQRMQVVQIMAPKDSTIAQVKDLVIVENQSPYLCVSSFHLAIDGKELDPQKTLGEYGITEQSQIDAIEQNDHLLHRDDERPRDWTVDEITAEDVKRSPYKEMEMQPLQNLAPRYEARPKGYFGRTYYSGMKQSS;> MRRVRDGLFLSHPSSALQCSVAVVSTGEFDHPPFQFRQRHTFNTTPLHDANRFGGRTAYLREIGPVNIKKQGRRFKKDPRTVQFNVDVWCAQQTLRKRWKQRDWEVIEIPFRLVPREQQRVIPELYTDIPQMTDPARNDFSNIRNKVYDREELQGVLFPAAGAMLYPPLQRVDKQAMTLDKYL;> MLRFTHRALTATPERFSVLGTTHPKPKRTGFGRNNKMRSKPSDNVAWYDKGPVEWLPRPVRLTYDHLDQLQQWTMRATLDGRTEEFNRIRDLHREWSQHPLMPVLGDVEPKFPLNLFKQNHRAKKRFLVRWHKANTPANWLWMPRGPTVVTPLHRTNPTQYPENWKQMVQRKSGTGTPS;> MFHRAFVSSSDLTGCTIALSSVCTQKRYWAKPKKRPKVGQGFHEKAQKWREEYLLDRHRALADSLRAYVEFSTSKRVEPWDARFKPFDRIEKDGVYVLMRYMMEEKLQLCNYHHRPVKRLFCNIGLMGPQITTKARWKPYRFATNPAGTSKAERMYQRDKTVYTHGHND;> MLRSTLTSLNTFLTSSVATPPISVIRTGPKWWAHPERMVRQKLMYFTLGVDQLPLRRTAVIQRDLQRFHMCKPPPRVGDSTGYKRSRAAQLNTWYRRIQYQEYHMQHLFTRHVWGLLRVYPGNTTKIQGKADDGYVGYDSVPFHRYNRAPLPFPARELYERRK;> MLRRSILFRMKYADLELTTRGEFPHGMKEPAFVKKLDQNIPWYFSTYRSMYHWPITGDNWSDLNEAEKHHDLHMFYTLAWWKLGEGIFGVDEDS;> MFSLTQTWLIAHWYCGHKFRHRFMRDKRFHPSLQASHDARNRFSKRRHFKTNRWNYQQAYRDMP;> MLRGWHPNSSAMQVGMRHITIGGRHSRGGFRQPLGKHPQVKQGTVEGVPRRIPGTTKVTYTNKKGRTFSFSVPVSELTHPQVTLESAAGTWREMDTSFCELGDIEDDMPSPVDECLRGGSSLDKRLIQEVRERFVSFCREYVLMDTSGMKSTILSTELNAGPDYEHYDRRLRRKRHWLAIRHRFEDVRYVIWPDVVEETARGDSAQADVSLTNPSLTAGEMLEALLWLDAASTFCVRKVHPSDLGDKSEFLPLDLQREVEVVACHARRDLDFFDPSATSLEQFTACAALCVNHRVPFSLFFPAQDVCGDASVSTGQCIVANAPSPHTALGAVRIMALISEGSGSDIGKTIMFSDAFGAVTRFGILRGLSRVMSVEAFGCKDALENVNESELCIILHFCAEVREQNAAFFRRYEASEEDSDPQQVSFLAKYQQLSQIALARCKRLLYHPDSPRAQVMSEDGYIPLVELQRHAEGTNKAALIHYNLGIRSAQGMRRVALGAQSSARLAELVSRLEEASARVSGNTLVNDLVHHLSHKAAAGKMSLTLREVNTLLPLLSRMRRESPNGALDARFDRVFNAIDTAIGAAMRHNCTLDELLDLAEGLAACEMVPSALKQVEMVLIRSVMMHECSPMHLRRMLQAMFTLMRTSVPQVLLQSVASRVADYIKEASHMDSSSSNGGGDEKVKNHEECEQLLELLVVLGKCGYGALPGLVTIYWEAQLIDSMQLNPRLRCSYASLLASAAFALKKHDKRAWEGLADESHRLFMEYTRCNKENDIGRFAECVTGLAVLTQIKDNTNSSDVAFLKEYLSATSLELKSCEVIRVQELTDLLGRTLEWSEALGVVAPDVVIQLEKALFVMLENVSHTAPGVGIPDELVTAACCLVDMSSASLELRKAAAGVVGGAIVHAEEALETLRSGAPTQVRPGHSFDVAALASAERENVYKNSILQYCAALQRSGMSTHVEELWS;> MYKKALHSFFLKVHPDFFHHNRSQQTVNESSVARLNELLSWAKAFKSGHLQPPPSSSFTLTFYRKPDDNMGNGETRREGSGSPVSSLVGRSMGDGSLSPTIIQSTFELPSNFAPSDNHRGTVERAVNKFLRDLLRRAACIDSVTESISEAEDATAARAEAKPLRRRPRGSQHRGAPTGPKSLLDEAVESMTVQWSLTPAPTLQELIEADQILFSRDLSPLQSAAALSTLQRHLGELNYSAWESMPVIVSNQFSIGDLTGTITIPWDFTPEQFHSFMAHNEKGVARCREVAIQYASTIEQLIAELCTALELDDILVSCSHQDALRLMELLHRNRELLIQYGLSKLTLEVGNRHATRANGVVIINCSLTSEQLRPWLKAISPKLPLQQRLYELSKQMLESTLWHLKEFRTMVEPGGVDAFSNDCTYAERLQWSKELFRIGPSLAPWDWSEMTFVLSPDVDIDWANGLLALPYNFDGDALVRYVEEVQQEAKSRKREELLAASAMQREEEERRRKQQHDEELMVECQEKGERSGDDSPTVAERMRHLYRQTNPHMDEYLASSNSRVDTLPVERPLSHAVTFNSDAEAEDQLKWEGFYAEPYVDQAPTSDIDDMAHTFMLTNRWHREEAAKKMLDQLRGTYGKKSRRFEYQKMGDVLEINNAKVQPKGFPTLTRGIKPGC;> MLSHAVPRLRLAAAAVKAAEWYAAENRRKQKGGDVIREKVDCTAPLWFDDTEQNLLAREQHVRSPAYRELHRPALTNAAMGLYGGEPGFEKAHRVWVDPDRPHIKHIYNQTALARNLRYARYGYFKRDMHLLDVDKLVRHARLLPTPGRLLTDFLYQRVPLPDKSCAALIRYQRQQIEMLEVWGRHASFQCAVEMFERMIVTNIPPVEVGVETHGEMVLCAAACGKWEEGWNVYANRARELEKESPESFILNTFFFDALLTLCVAAGRVSEGIDTLEEVIKRNLRPRGTMLNKAMILYSILGEQMSKHEASRATSEGERSYLCEPEEVEKMGLEVWSLFDFYQLPRTTASIEAYMRMCCAFNKPTLVLKAQGFADASDIRLSIECFHWLVYAIRGVAGFGDYVMDVLSQLRPRGLTPDFVLFTLSFMYCALQRDGELALAIFDQHFVHQNMNPTPEMVLLFIQACSNCEEPTAVMLERSETLIKRLEAVGSSVDLISPIYDQFLELCAHLGAVASGFSALKRIVGFGKPLTTRMINSLLLANSNAISSNGSLSMTEELVGFFTLLKIRPNADTEICVNLCRDAFGESPVVNDFIKVIGESLQGDSEKGEAPQYDEDIPVIQVPPHELRQLRTEWKLSPRDIVLRRFGQHTKPPGKAALDVGSMRGSVIPFGRSPGEQLV;> MTGPTRALFLSSGINLGRLRLAEQFSSMNGWQSKEDPAFDAYVKERRRKENYEAFDQRVERGYAAAAKLHKAEIQNAVKRRLKSSGAKFTAETLREMSSAVTERLAWLRDVWAQIDADYRSGDSARQETAAQEISAALRGEPNDYMRWVYETKRELRFAGPVGRRAIQEELQAAELPEVLDEEVNRYHDLKLNMMEIEREVKAKYGVAGQQHWAELQAAKDEEYIQKLDEAAEVYKQLLDQSARLDESRRSELQRSYVERVHQAQVRFKAAMELEGQREQLIEAHQAMKEERMRTEREKRRQLLREAAELRAQGKKSADVLTALKERQLDANAKRQAEYELKECEDILKRKSEMLDMIAHFKHDVEEREGREMLQRQKSDEERQVNVFGFYEEVGVEDGLSISSEGTTSQGGSSGLGTVSTSTSCAKSADSNSSAQPSQKLRKEELWKVINADTYEDPFRTVHQARLDAVKTYDPAYARTFPLNLVLGRKYSRQGAGEMAAGNETDKQILQKGNNILYSFQWGLNNGTVHDLDADGGTDYFMDGAFHVRDKETGDIDWRYEKKRGGPVFRGPKFYRLGAQREAADPGERAMDPTPYTSTPREHKWRSS;> MTDPVRRDPTEFLRVLRRMSRTTSWQKTMLFASKGRMVGYRLTREHYNTVLFSQSLWGRALEIVRVVRAMQEDKVQPNGATYYYIVNGMGNADHGWNYDFRINRRLEKIQHWRVALEALEACEANGFDSTDTMHNSALITLVIPGFNRWQQASLLLQRMLREDRRMHPTMVKFYHDCLVRNNRPREASSLMRLAAERGVHGYEDKWEADVYKGRPLDSEVMNESEGNGLRRQASSLAFASLMLRGDQRPLPENLQALLEEETTRNIEAERSVPVPFSAGLHATEINSVFRPRVYRQLWYKWQHIANRYRPTAALKRRQLAPRDSPTGIPGFYRI;> MKRIFRSSVRVGAALPLGAVVPAIFYCNGIRIMGRQYTHDTYRPFGDGYKEVRGTAPTDECNLLFASLNDESLPLCEDSGNVVNGQLVRASALVDSDALADSQELVDVAIEEDRREEEDNSVLLVPXHEEQNSVTKKQNEGEDVTTRCDHLFSVVGCPTTVSTATSGIPNTPSRNYLSEQDALYLSPTTPEEARVPSALCPQLSACVMVVFAANDMRVHDNYALALAATRAEAAGGLPVIAVTVVDYRMFAQPSAVGGFFRQSPMRARFFLETLAALRYKLERELRIPLLVRCGRPEDHIPRLVVECGAIDVFLTTQYAPHEKEVHNDIVEAINQRRWVSRDPTAGYKAIEHDATVVHPFGATSASTKVGVKESRLTAAPVAHSVWQTTLVHIDDLPVPVASMVEGERWYHDDVTTANIRPTAAFDRCINRLSDLPARGDLLPTTGELSGLEPPPLYRGRAPTLVELGYGSPEAFIEEEVIATQSSHPPGEDAAIERVLDWLMDGGMTSMLRYGRDRRTNTKMYSQRLSRLSPYLSCGALSPRRFYEELRRFTSEHLRDNFVQQQYREALLRLSRRDYWHWMGLRYGPLLFYEYGPRPEHTDDIADWRHDPKIVQKWCAGLTGIPFADAAMRELTLTGFVADEGRQGLIWLLSRGYGQDWRLGAEWLERCSIDYDPFVCYGNCAYYSELVRDDFGETVRNIHWLAHHHDQTGIYVKKWLPQLSKIPPVYIHRPHVLTERMQAMHGVQLGKNYPYPLKLWDGAQYTLSSEHLTTYFSEGSQWHRKAKNGAGGSGYAEALRHGTVILEPHQLQSSAFGELEHGVMHTVPVVKDDTAGRGQHNRSLTASDE;> MSKSLQRALVFSGQGAHRRGMATEYLRIPAVACLWERMKGSMEQKYGISLQDIITENPTRLYVYNDAYDVAAICERSCQDGGSVVESTPKQKLISHPQGVLSLTSLTQPCMLAAHMVSLEYLKETRGYSVESSEVIAGHSLGEFSALCALGVLSPEVAIDLVYRRGALMEDAVKHSSQSNEGHLMFACNPQRAKLCVEDPDLAVDQLHIFVELIARNLSTTASFIEVVNYNISYEQYVVVGDPIALSALGKCLDPQFRATSCGSSATLDNIVRTAVSSVLQDKQEGITMNPNTGPAPDFVTSCARKYGIRSTFRRFLRGPDDGYTPSLEELTHLTLQEDGRSGLKKKSWFIPLPLSIPFHSSMLRRAMDLFLPVVRDALPDEETMRSFFCIPQCGGSDXGPSSRCASEPKKPVWLTNLTGTAFRPFDVDFQRDALDAMQSMNVGEIRHNGRYHTNLVELAFKNGMDTSSVRDMCAAVLAAQLAHPVQWIDVMDSAVFQHGVREAHEISPVRTVADMFKRTVFRGKTSDASVGEAALDIVTRCLPSEERFL;> MWQRLRFDRLSSSVRRTNLNPLKPCAALTEQRAELRNLHQYPTARHKSLVKDRLRFARNWWLTGGNNYELVHEVGHEREATECFAEYAQDSSRDVYLMSTNRLSDLPPGDRLKAIVGLMRSRWEVKDANRGYDKAKLLLQALECFSEMKASGQIGDFNSLPEPDQDTFLQYVEGCSRFAQACSHSHPDAVRVLLRAAQICEEMRCVEKRDEMIQVTEAAANRMDRAYAFSRPHDTLRAAPPSLHENEDCVRLKNTEELRRRFGNTAPHVLEKPKRVDCLRIHRNRPLLLHPMKDNNKLLELSKLPARPEFDSWTSHQT;> MRGSLPLLFNPVLPPSTARLRLLTYPMALAQPHATVPLIQPTIDGTHDGRNGATVSLRTQARMHGTADGTMATAGDSSQNNSVMDSPRWLRNPDELCVAALRRSRDVNKINSYVATYKFDDPQWAPLLLPEVTLRPQVNSTGDKPNGGNEAAADVVSVGPSVSATPESTPPPPPSSSSSSPYSCPADCVSISHNKMIMLECMSRHVNFSLRHIVQKGHGIYLIYHAQHSILQPKGLVEQSFVTCSFGIRGERLRTDIVHVGPIDAADVMELQPSEGHDHPRCCFNLYQKSDVRRGVIAVSQVEGYGTWFQRKPMLWQRSRRIGALQSQLGAFAYDLVDPHEVGKWRDCEVSLLAPHMRFFRNGLNGAEAVGIIASSQVAQQRRLYLGEFEAPAITALDAVQQLAHASALRCKLVTPVVDPNGVGGTGSGSLGDENMDKHIDMETLLPLSWATRTPPPYVPLEADLPFKLQMSRPTVFAESHQQNQAYPTGGTVGSPFVRGAPMMMFEYNMHQGVDHYVYDDAPSARPMKWWSQKSNMPYSGYMYFARSGLVDRFTPSEDIPNPLEPTSKRKPLHAVVPPTKVVQERLRKYRRKQQEGHKQRRRASSGSGVSNEPDAVNRQESVSRGTCE;> MQSGLCHCVRRVAALGSVANLHHFTNLPSGFSVWTSRRWQSQSSRGQPGLQWQEGVVDPRYSSSGNMRRFNPDTVAHYVKATIQNDRREMGLGEVYDWHEFAKDAVYIPTRSGPLWVGSDDPRCAKFMRRRSKMQKTPQQKARPKPGPDPAKALEDHPLREYFTTATNLRDPLSTANNLHRAGLIREYDIKYTAAKVRYVPRPPVVSIMGHVDHGKTTLLDYLRKTNVASQEAGGITQNVGAFQVKTLGDTLVTFIDTPGHAAFTTMREVGATANDLIVLVVSAVDGVQPQTKEVIELAHKSGIPFVVACTKIDRQPRVENVKQQLRDCNVELEEDGGDTQFVPVCARDGRGVPELLEAIALQAELCEISTPKPSRCEVTVIETNGVNTTTEVAGIVRCGKVRAGQVLVAGMTYAVVRKVLDEHGQIIQEAGPSQPVVLHGFRVHPKPGSILLQVSSESHAQKFYHFMKEVYQAEGRREDYLQLLNQEQHGMLYARKPDNNLVRTYSTQAFVLSCKAATFGMLQALMKSIYEIPRLEGISTEIKVTEVGGLRDYDVALIGSSGQPGCILLYGGCKDTNTLDVPNHVTVIRFNVLYHGLEALKETLVGALPKITKIRVTAEAECLQVFRASQAGKSGNAGGMRVTKGTIIAAHLTFRVCRKAPLVKGTAETDGVSDNEGDGDEDMLGHRVVVYEGQIKELRRFKELVPSVELGLECGVIMQDEFQFRTGDILQQYETYEEPRDVAEEYQKAELREKIMRDTAAAEALLAESTGGEDKPTEESEVKTTI;> MRRSGRGSAVRWSSLCKCQCCLYRTPLGGTYFEQALPRSLGARQGKGVLSTVNTALSRKALKRRQSLPRKKLNVPLTAEGLKERLKQLSAEERELSIKNNTEECDEPSPNEFTTTHEARVALARVLHHGENAGERKEVAMRIPSFCRSPAVSETQSIVVDDKEGDITNAAVHVGCSVLGSDLDHLERDMIRDYHQRGKKLPTFDNIYRTLGCGRKGTSVSDTEPEDENSSGAIQSECGLGDAGRRGTVVVAPSHLHHSTPPTKGRSGEEEEEGGCFDTNTLPADANPHFPPGACDNEVLAPLSGGCAASEQTEITDTASFIPSNSRLSTAVYDAYRQRPADDRLVVLRGTDFWDNEENRARLQELTDYAEEDFAREMLMEGAMDTSEVGYSTNKVRKETLLYFQAHPINEMIQEPFARVRSILPSDGGPEVHFPADDPDTDVDIPTAQARTMARELGLDLIRVGTLYTPINDRRVVAVCTIADHREHMRDMIRFKIKKLGVQRPPTKEGIEVPFRGGTHPHAVRFKSIGIAKHLLLGHVVRINLTDFGTVREGFPVFGSILDEVARQALQLHAYHTAGVVRANYNEVYCYLYPSTGRSPKSTVLHPTQEQLATVRDRCLLEREREVYFDGLYDKKTPRERLTYMRKLQDGTAWADRDDGLSLQRQRDMKVMLGYLPKGNHELYAARGDVNVPAPFRASHPTSVDRWTHPQESNLEQAARGSAVLAKRLSMTVSEMHDRQETAENPATLDRFYYRIQGPALEAGELKEALGLKGNRKRLPRRAPGWATLGMEKVSPQEPGHAAK> DYEIQRERIELGRCIGEGQFGDVHQGIYMSPENPALAVAIKTCKNCTSDSVREKFLQEALTMRQFDHPHIVKLIGVITENPVWIIMELCTLGELRSFLQVRKYSLDLASLILYAYQLSTALAYLESKRFVHRDIAARNVLVSSNDCVKLGDFGLSRYMEDSTYYKASKGKLPIKWMAPESINFRRFTSASDVWMFGVCMWEILMHGVKPFQGVKNNDVIGRIENGERLPMPPNCPPTLYSLMTKCWAYDPSRRPRFTELKAQLSTILEEEK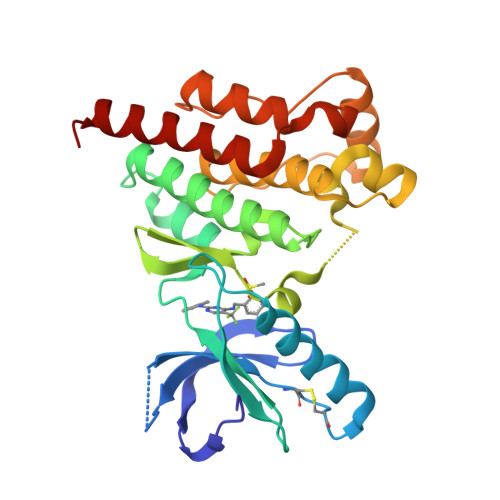AQQEE> MSKNEEMEGKMFIGGLSWDTTKKDLKDYFSKFGEVVDCTLKLDPITGRSRGFGFV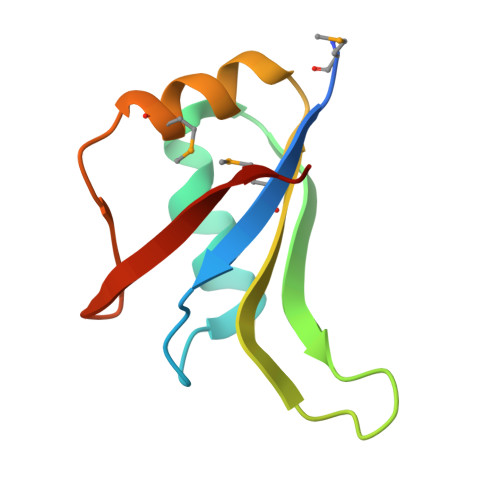LFKESESVDKVMDQKEHKLNGKVIDPKRAKAM(2S)-2-HYDROXY-2H-CHROMENE-2-CARBOXYLIC ACID | C10 H8 O4 | 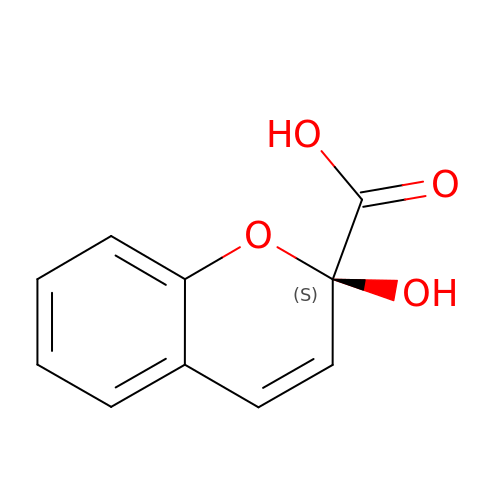LGYIZQLNYONEFJ-JTQLQIEISA-N>MTMITNSRGSLSDGALSTDNAAGVNLFTAYPSSGVSGSTLSLTTGTDTLTGTANNDTFVAGEVAGAATLTVGDTLSGGAGTDVLNWVQAAAVTALPTGVTISGIETMNVTSGAAITLNTSSGVTGLTALNTNTSGAAQTVTAGAGQNLTATTAAQAANNVAVDGGANVTVASTGVTSGTTTVGANSAASGTVSVSVANSSTTTTGAIAVTGGTAVTVAQTAGNAVNTTLTQADVTVTGNSSTTAVTVTQTAAATAGATVAGRVNGAVTITDSAAASATTAGKIATVTLGSFGAATIDSSALTTVNLSGTGTSLGIGRGALTATPTANTLTLNVNGLTTTGAITDSEAAADDGFTTINIAGSTASSTIASLVAADATTLNISGDARVTITSHTAAALTGITVTNSVGATLGAELATGLVFTGGAGADSILLGATTKAIVMGAGDDTVTVSSATLGAGGSVNGGDGTDVLVANVNGSSFSADPAFGGFETLRVAGAAAQGSHNANGFTALQLGATAGATTFTNVAVNVGLTVLAAPTGTTTVTLANATGTSDVFNLTLSSSAALAAGTVALAGVETVNIAATDTNTTAHVDTLTLQATSAKSIVVTGNAGLNLTNTGNTAVTSFDASAVTGTGSAVTFVSANTTVGEVVTIRGGAGADSLTGSATANDTIIGGAGADTLVYTGGTDTFTGGTGADIFDINAIGTSTAFVTITDAAVGDKLDLVGISTNGAIADGAFGAAVTLGAAATLAQYLDAAAAGDGSGTSVAKWFQFGGDTYVVVDSSAGATFVSGADAVIKLTGL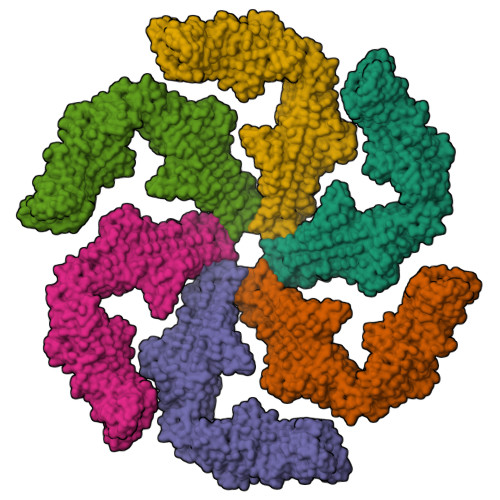VTLTTSAFATEVLTLA[6x]> REFTIDFSTQQSYVSSLNSIRTEISTPLEHISQGTTSVSVINHTPPGSYFAVDIRGLDVYQARFDHLRLIIEQNNLYVAGFVNTAT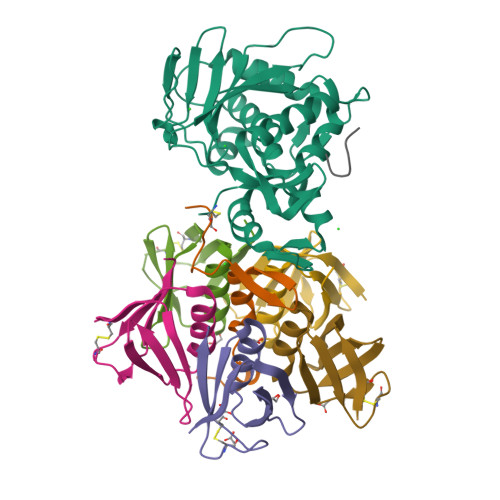NTFYRFSDFTHISVPGVTTVSMTTDSSYTTLQRVAALERSGMQISRHSLVSSYLALMEFSGNTMTRDASRAVLRFVTVTAEALRFRQIQREFRQALSETAPVYTMTPGDVDLTLNWGRISNVLPEYRGEDGVRVGRISFNNISAILGTVAVILNCH;> PECQITGDRPVIKINNTLWESNTAAAFLNRKSQFLYTTGK;>ADCAKGKIEFSKYNEDDTFTVKVDGKEYWTSRWNLQPLLQSAQLTGMTVTIKSSTCESGSGFAEVQFNND[5x];> GFGLFD>QPDSVSIPITCCFNVINRKIPIQRLESY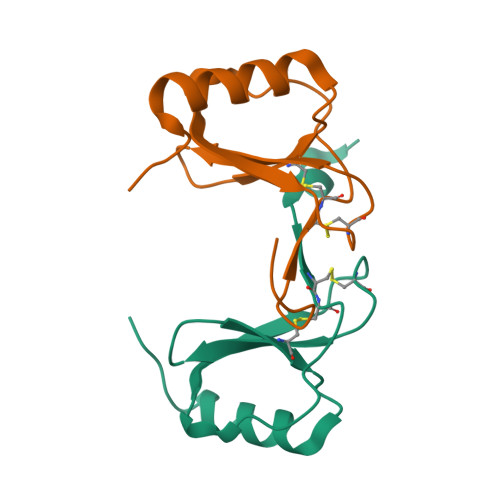TRITNIQCPKEAVIFKTQRGKEVCADPKERWVRDSMKHLDQIFQNLKP[2x]>MVTAHFVLIHTICHGAWIWHKLKPALERAGHKVTALDMAASGIDPRQIEQINSFDEYSEPLLTFLEKLPQGEKVIIVGESCAGLNIAIAADRYVDKIAAGVFLNSLLPDTVHSPSYTVEKLLESFPDWRDTEYFTFTNITGETITTMKLGFVLLRENLFTKCTDGEYELAKMVMRKGSLFQNVLAQRPKFTEKGYGSIKKVYIWTDQDKIFLPDFQRWQIA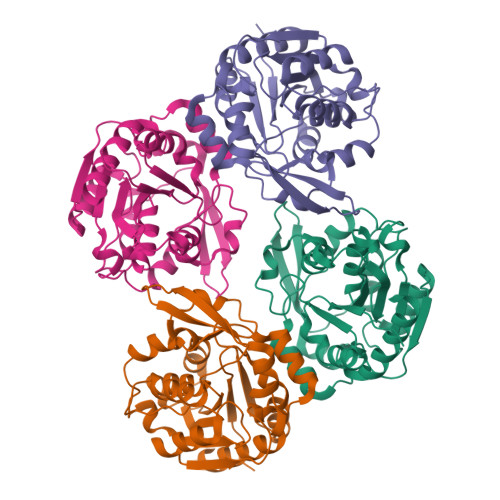NYKPDKVYQVQGGDHKLQLTKTEEVAHILQEVADAYA[4x]>MGHHHHHHHHHHSSGHIEGRHMKKPRIDMHSHFFPRISEQEAAKFDANHAPWLQVSAKGDTGSIMMGKNNFRPVYQALWDPAFRIEEMDAQGVDVQVTCATPVMFGYTWEANKAAQWAERMNDFALEFAAHNPQRIKVLAQVPLQDLDLACKEASRAVAAGHLGIQIGNHLGDKDLDDATLEAFLTHCANEDIPILVHPWDMMGGQRMKKWMLPWLVAMPAETQLAILSLILSGAFERIPKSLKICFGHGGGSFAFLLGRVDNAWRHRDIVREDCPRPPSEYVDRFFVDSAVFNPGALELLVSVMGEDRVMLGS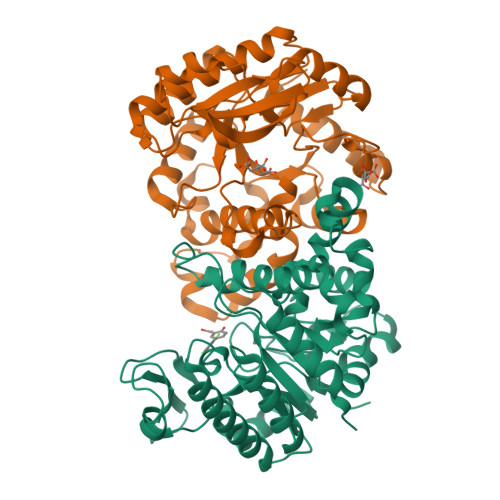DYPFPLGEQKIGGLVLSSNLGESAKDKIISGNASKFFNINV[2x]3-chloro-5-[2-chloro-5-(1H-pyrazolo[3,4-b]pyridin-3-ylmethoxy)phenoxy]benzonitrile 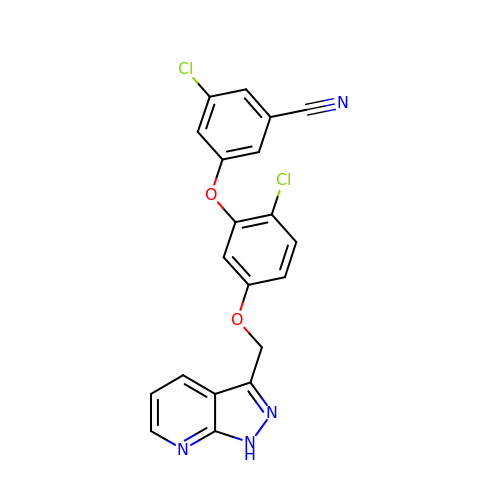| C20 H12 Cl2 N4 O2 | SVMHTBVIPYVDIL-UHFFFAOYSA-N> MFPMDTKTNE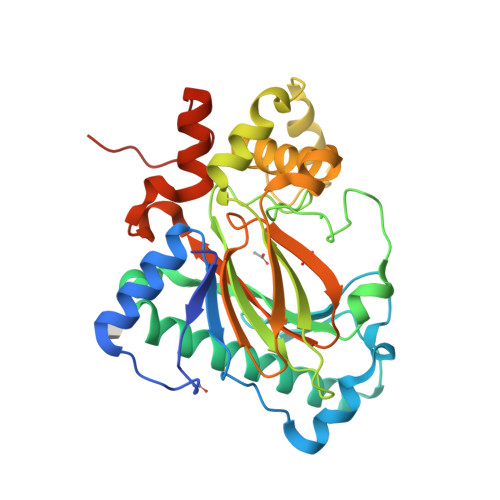QPIIQFDAESWEAEFTQEIQDKAIEGLESGSVLFFPKLNFPLLTEELKFLDPTWVSGAKNISYDPRSATLKGVEGKSEDLRLLSGLLKRYAEKTAAFLHLLFPFYGSSLKIARTSFRPVEISGRATSARKDDTRLHVDAFPSSPTGGERILRVFSNINPQGKPRSWRIGEPFQNYLNHLLPQLSPPAPGKRFLLYLFGITKGYRSLYDHYMLELHDKGKLDLEYQKNSPQVAFDFPAGSTWIVFTDQVLHAVDKGQFLLEQTFHLKVNALKHPEKSPLKLLETALNKKLVSSESFKLAAALEHHHHHH> MHHHHHHQHQHENLYFQGMQTKKNEIWVGIFLLAALLAALFVCLKAANVTSIRTEPTYTLYATFDNIGGLKARSPVSIGGVVVGRVADITL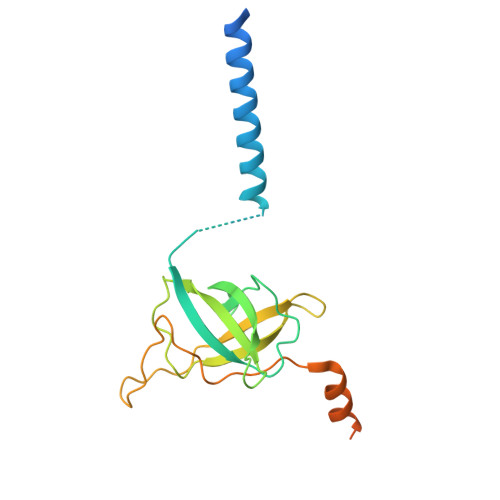DPKTYLPRVTLEIEQRYNHIPDTSSLSIRTSGLLGEQYLALNVGFEDPELGTAILKDGDTIQDTKSAMVLEDLIGQFLYGSKGDDNKNSGDAPAAAPGNNETTEPVGTTK> QPIFLNVL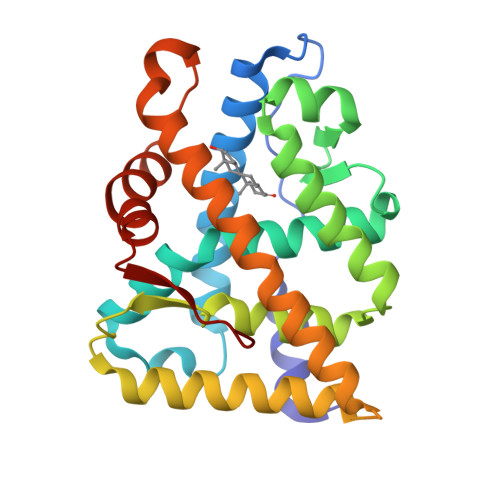EAIEPGVVCAGHDNNQPDSFAALLSSLNELGERQLVHVVKWAKALPGFRNLHVDDQMAVIQYSWMGLMVFAMGWRSFTNVNSAMLYFAPDLVFNEYRMHKSRMYSQCVRMRHLSQEFGWLQITPQEFLCMKALLLFSIIPVDGLKNQKFFDELRMNYIKELDRIIACKRKNPTSCSRRFYQLTKLLDSVQPIARELHQFTFDLLIKSHMVSVDFPEMMAEIISVQVPKILSGKVKPIYFHTQ3-[2-(4-methoxyphenyl)-2-oxoethyl]-5,5-diphenylimidazolidine-2,4-dione | C24 H20 N2 O4 | 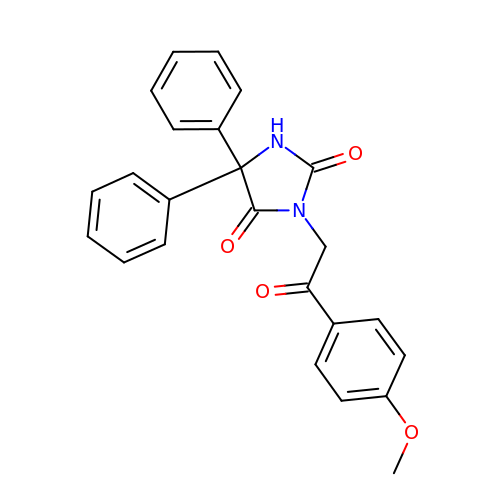BZIXIEVSXWQXTK-UHFFFAOYSA-N>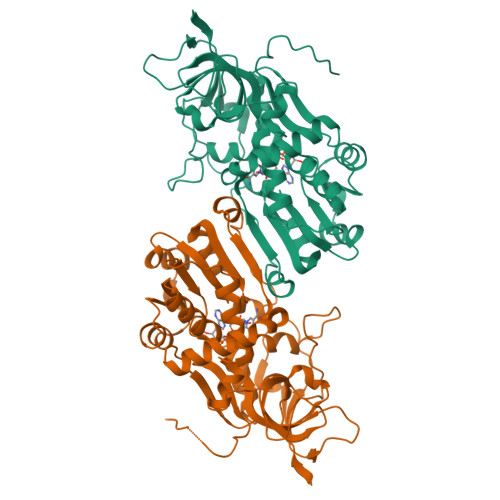[2x]MASAEDVVVVNKQVLLKHFIPEGAPKETDMELVTTGTIRLRVPEGSNAVLLKNLYLSCDPYMRMRMTKHEEASYVDDFVPGAPITGFGVGKVVDSSHPDFKTGDYVWGLIGWEEYSLITKPQGLFKIHHTEIPLSYYTGILGMVGLTAYVGFYDICSPKKGERVFVSAAAGAVGQIVGQFAKQFGCYVVGSAGSDEKVNLLKTKFGFDEAFNYKKEPDLTKALKRYFPEGIDIYFENVGGPMLEAVLHNMRIKGRIAACGMISQYNLEKPEGVHNLFLIVGKRIRLEGFLVFDHYGSYPEFEEKVVQLIKEEKIKYLEDIVEGLENAPAALIGLFEGRNVGKQVVVVSREKGHHHHHH> AEAPTTSTTSA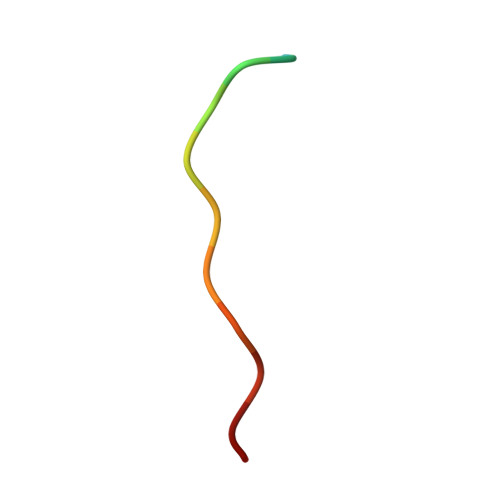PK>GSRKIIHVDMDCFFAAVEMRDNPALRDIPIAIGGSRERRGVISTANYPARKFGVRSAMPTGMALALCPHLTLLPGRFDAYKEASNHIREIFSRYTSRIEPLSLDEAYLDVTDSVHCHGSATLIAQEIRQTIFNELQLTASAGVAPVKFLAKIASDMNKPNGQFVITPAEVPAFLQTLPLAKIPGVGKVSAAKLEAMGLRTCGDVQACDLVMLLKRFGKFGRILWERSQGIDERDVNSERLRKSVGVERTMAEDIHHWSECEAIIERLYPELERRLAKVKPDLLIARQGVKLKFDDFQQTTQEHVWPRLNKADLIATARKTWDERRGGRGVRLVGLH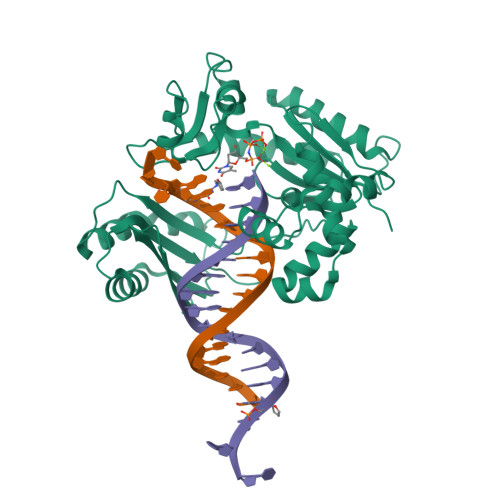VTLLDP[2x]> MEKDGLCRADQQYECVAEIGEGAYGKVFKARDLKNGGRFVALKRVRVQTGEEGMPL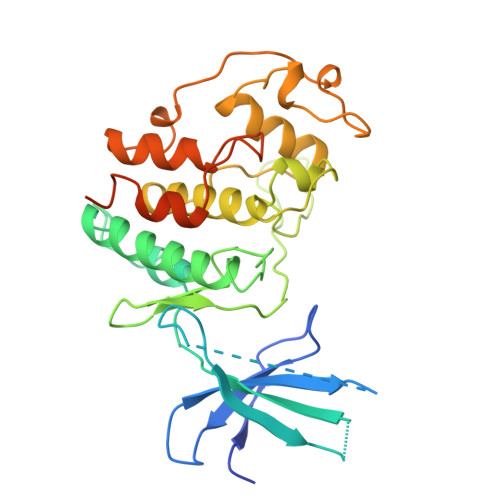STIREVAVLRHLETFEHPNVVRLFDVCTVSRTDRETKLTLVFEHVDQDLTTYLDKVPEPGVPTETIKDMMFQLLRGLDFLHSHRVVHRDLKPQNILVTSSGQIKLADFGLARIYSFQMALTSVVVTLWYRAPEVLLQSSYATPVDLWSVGCIFAEMFRRKPLFRGSSDVDQLGKILDVIGLPGEEDWPRDVALPRQAFHSKSAQPIEKFVTDIDELGKDLLLKCLTFNPAKRISAYSALSHPYFQDLERCKENLDSHLPPSQNTSELNTA Nalpha-{4-[4-(4-aminophenyl)buta-1,3-diyn-1-yl]benzoyl}-N-hydroxy-L-histidinamide | C23 H19 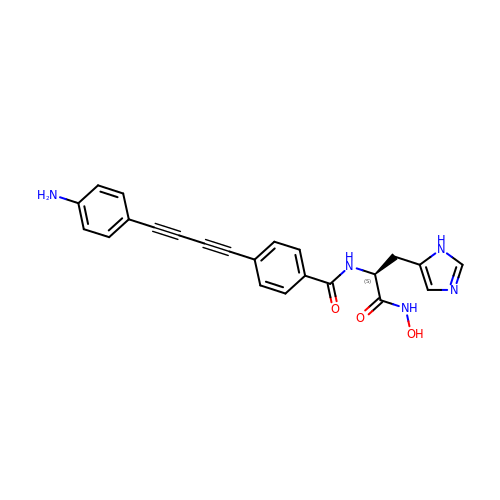N5 O3 | AEXNUUIGAXOZGM-NRFANRHFSA-N N2-(CARBOXYETHYL)-L-ARGININE 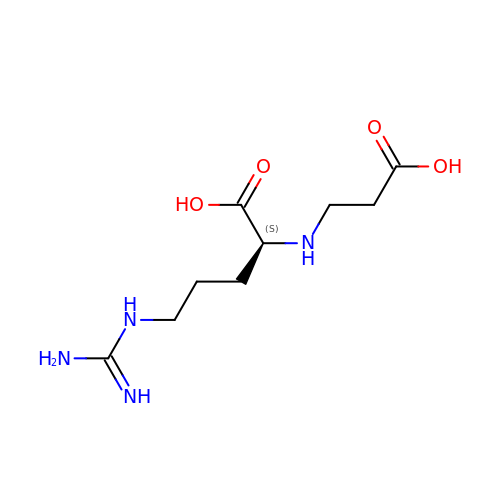| C9 H18 N4 O4 | OHWCFZJEIHZWMN-LURJTMIESA-N> IVGGYTCGANTVPYQVSLNSGYHFCGGSLINSQWVVSAAHCYKSGIQVRLGEDNINVVEGNEQFISASKSIVHPSYNSNTLNNDIMLIKLKSAASLNSRVASISLPTSCASAGTQCLISGWGNTKSSGTSYPDVLKCLKAPILSDSSCKSAYPGQITSNMFCAGYLEGGKDSCQGDSGGPVVCSGKLQGIVSWGSGCAQKNKPGVY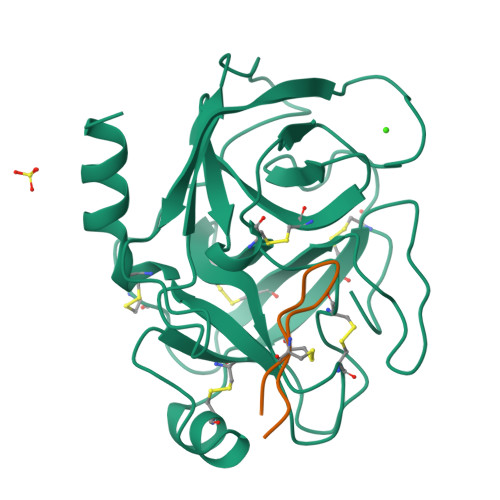TKVCNYVSWIKQTIASN;> SSEPCCDSCRCTKSIPPQCHCANIRLFCYKPCESM>MGLMKFQLFIQPKLDVLQGNIVEYEILLRDDSAVPRFPLSELEAVLADEELYLAFSEWFSEAFLDVLKKYPNDRFAINIAPQQLFYIETLHWLDKLKSESHRITVEMTEDIFDVPGHKRHLNANDKNAF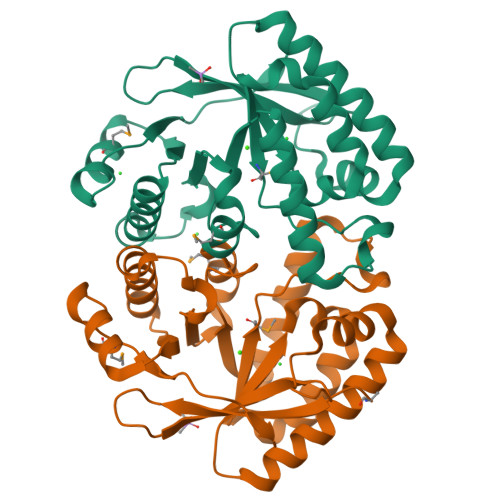ILNKIKVIHGLGYHIAIDDVSCGLNSLERVMSYLPYIIEIKFSLIHFKNIPLEDLLLFIKAWANFAQKNKLDFVVEGIETKETMTLLESHGVSIFQGYLVNKPFPV[2x]(2Z)-2-cyano-N-(3'-ethoxybiphenyl-4-yl)-3-hydroxybut-2-enamide | C19 H18 N2 O3 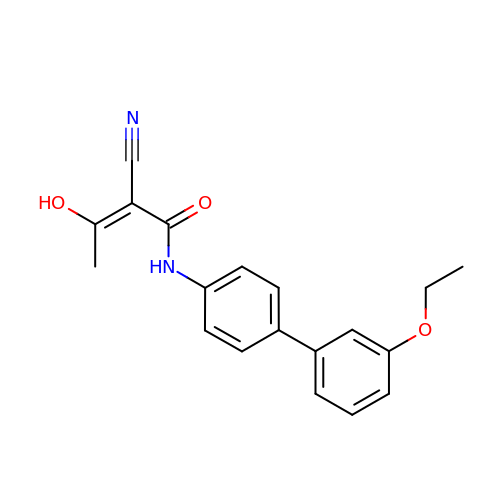| RPILZQUCBKIPAZ-AQTBWJFISA-N>[4x]GSHMTDLNIPHTHAHLVDAFQALGIRAGQALMLHASVKAVGAVMGGPNVILQALMDALTPDGTLMMYAGWQDIPDFIDSLPDALKAVYLEQHPPFDPATARAVRENSVLAEFLRTWPCVHRSANPEASMVAVGRQAALLTANHALDYGYGVESPLAKLVAIEGYVLMLGAPLDTITLLHHAEYLAKMRHKNVVRYPCPILRDGRKVWVTVEDYDTGDPHDDYSFEQIARDYVAQGGGTRGKVGDADAYLFAAQDLTRFAVQWLESRFGDSASYG

Specifically, AAC(3)-IIIa and its fellow isozymes catalyze the transfer of an acetyl group of acetyl-CoA to the 3 position of the aminoglycoside’s canonical 2-deoxystreptamine (DOS) ring. Here, we present three crystal structures of AAC(3)-IIIa isozyme (isoA) from Pseudomonas aeruginosa in complex with 4,5- disubstituted neomycin and 4,6-disubstituted sisomicin and gentamicin. The substrate promiscuity of isoA is due to its tripartite active site, which can accommodate a variety of aminosugar ring attachments, this architecture was first described in APH(3’)-IIIa and subsequently found in isoB. The isoA crystalizes as a homodimer, with four molecules in the asymmetric unit.

Our structures of isoA bound to sisomicin and gentamicin are also allowing us to outline this enzyme’s specificity towards 4,6-disubstituted aminoglycosides. For sisomicin, the prime ring binds to three water molecules which can coordinate the sidechain of D170 and backbone ketone of G213. Unlike the double-prime ring for neomycin, sisomicin’s double prime ring is stabilized by a mix of water-mediated and direct interactions. D72 can form direct interactions with the 4″ hydroxyl and 3″ amine, while it is also responsible for a water-mediated interaction with the 3″ amine. A second water molecule mediates interactions between O-6″ and D211 and T212. Sisomicin interacts with one final water molecule at the N-3 position of the central ring, which is coordinated by the backbone atoms of D170 and I172. The catalytic efficiency demonstrates that while sisomicin and kanamycin are both 4,6-disubstuted antibiotics, they are the most and least efficiently converted substrates, respectively. Based on our crystal structures, we can deduce that the N-1 HABA substituent introduces a steric clash that prevents these aminoglycosides from binding to isoA. It is predicted that hydroxyethyl chain on plazomicin’s 6’ position would be able to be accommodated, as homologous 6’ amine of sisomicin is solvent exposed.> FAGTVSALASIGLGLLGKSSATPSVIKGIAQQAVGAVQANPGILEGAVKAIGSVGARLVGSIKARRARRRARR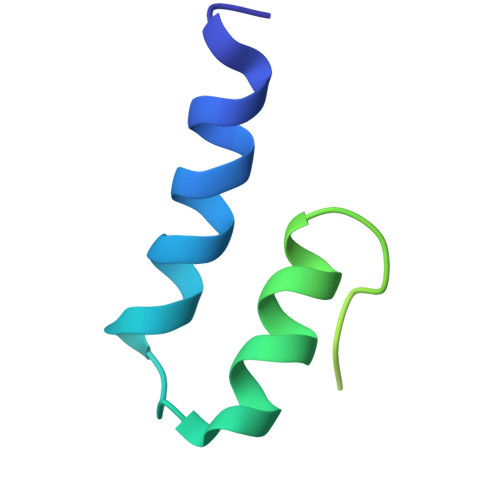AK> AFTTGLVYDTLMLKHQCTCGSSSSHPEHAGRIQSIWSRLQETGLRGKCECIRGRKATLEELQTVHSEAHTLLYGTNPLNRQKLDSKKLLGSLASVFVRLPCGGVGVDSDTIWNEVHSAGAARLAVGCVVELVFKVATGELKNGFAVVRPPGHHAEESTPMGFCYFNSVAVAAKLLQQRLSVSKILIVDWDVHHGNGTQQAFYSDPSVLYMSLHRYDDGNFFPGSGAPDEVGTGPGVGFNVNMAFTGGLDPPMGDAEYLAAFRTVVMPIASEFAPDVVLVSSGFDAVEGHPTPLGGYNLSARCFGYLTKQLMGLAGGRIVLALEGGYDLTAICDASEACVSALLGNELDPLPEKVLQQRPNANAVRSMEKVMEIHSKYWRCL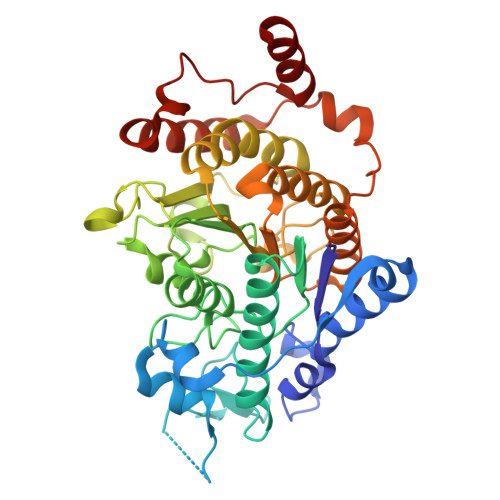QRTTSTAGRSLIEAQTCENEEA>[3x]MNPVTKQFQFGQSTVTLETGRIARQATGAVLVTMDDVSVLVTVVGAKSPAEGRDFFPLSVHYQEKTYAAGRIPGGFFKREGRPSEKETLTSRLIDRPIRPLFPEGFMNEVQVVCTVVSTNKKSDPDIAAMIGTSAALAISGIPFAGPIGAARVGFHPEI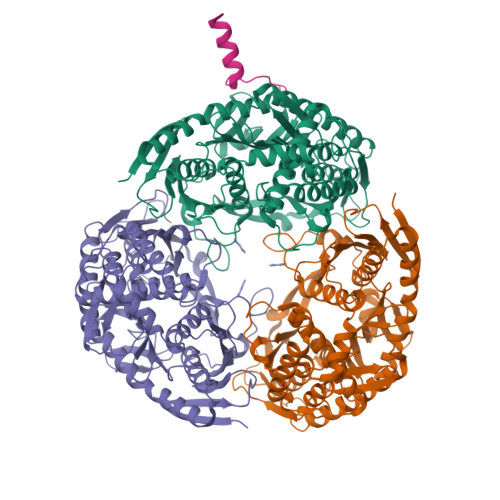GYILNPTYEQLQSSSLDMVVAGTEDAVLMVESEADELTEDQMLGAVLFAHDEFQAVIRAVKELAAEAGKPAWDWKAPAENTVLVNAIKAELGEAISQAYTITIKQDRYNRLGELRDQAVALFAGEEEGKFPASEVKDVFGLLEYRTVRENIVNGKPRIDGRDTRTVRPLRIEVGVLGKTHGSALFTRGETQALVVATLGTARDAQLLDTLEGERKDAFMLHYNFPPFSVGECGRMGSPGRREIGHGRLARRGVAAMLPTQDEFPYTIRVVSEITESNGSSSMASVCGASLALMDAGVPVKAPVAGIAMGLVKEGEKFAVLTDILGDEDHLGDMDFKVAGTDKGVTALQMDIKINGITEEIMEIALGQALEARLNILGQMNQVIAKPRAELSENAP;> VPANATGRALNDPREKRRLQREAER> MAFSRPGLPVEYLQ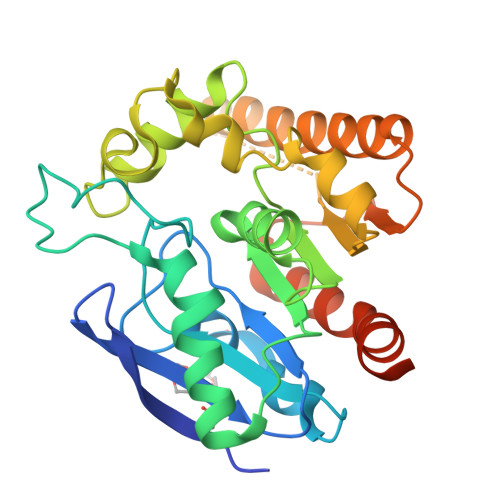VPSASMGRDIKVQFQGGGPHAVYLLDGLRAQDDYNGWDINTPAFEEYYQSGLSVIMPVGGQSSFYTDWYQPSQSNGQNYTYKWETFLTREMPAWLQANKGVSPTGNAAVGLSMSGGSALILAAYYPQQFPYAASLSGFLNPSEGWWPTLIGLAMNDSGGYNANSMWGPSSDPAWKRNDPMVQIPRLVANNTRIWVYCGNGTPSDLGGDNIPAKFLQGLTLRTNQTFRDTYAADGGRNGVFNFPPNGTHSWPYWNEQLVAMKADIQHVLNGATPPAAPAAPAAHHHHHH Naphthalene 1,2-dioxygenase from Pseudomonas putida strain NCIB 9816-4 (NDO) is one of the most well studied Rieske dioxygenases; it is an α3β3 hexamer and is the first Rieske nonheme iron oxygenase for which the three-dimensional structure was determined. The α subunit of NDO contains a Rieske [2Fe–2S] center that accepts electrons from the ferredoxin component, which originate from an NAD(P)H on a reductase component, and transfers them to a nonheme mononuclear iron at the active site. The catalytic domain of the terminal oxygenase is the well described 2-His/carboxylate center composed of a mononuclear iron coordinated by two histidines and one aspartic acid inside a large hydrophobic active site. NDO has a relaxed substrate specificity and catalyzes the dioxygenation of many two-ring and three-ring aromatic compounds to their respective cis-dihydrodiols.

In order to study inhibition of the activity of NDO by inhibitory compounds, we also complexed NDO with the known inhibitors indole-3-acetate and benzamide and determined the structures of these complexes. The structure of NDO in complex with benzamide was determined to 1.65 Å resolution. Benzamide does bind in one orientation in the active site of NDO. It was hypothesized that this compound should bind tightly with the heteroatoms near the mononuclear iron because the aromatic ring could be positioned between Val209 and Leu307. In addition, the amide group would be able to interact with charged residues on the wall of the active site, while forming hydrogen bonds to the water/hydroxide bound to the mononuclear iron. The N atom of the substrate forms a hydrogen bond to the water/hydroxide that is bound to the mononuclear iron. The O atom of the inhibitor interacts with the side-chain N atom of Asn201, which is 3.6 Å away, and the side-chain N atom of Asn297, which is 4.0 Å away. There are no examples of NDO catalyzing the oxidation of compounds containing an amide group and it is unlikely, based on structural evidence, that NDO would be able to catalyze the oxidation of substrates with amide groups that are free to interact with the mononuclear iron very efficiently.

> MNYNNKILVSESGLSQKHLIHGDEELFQHELKTIFARNWLFLTHDSLIPAPGDYVTAKMGIDEVIVSRQNDGSIRAFLNVCRHRGKTLVSVEAGNAKGFVCSYHGWGFGSNGELQSVPFEKDLYGESLNKKCLGLKEVARVESFHGFIYGCFDQEAPPLMDYLGDAAWYLEPMFKHSGGLELVGPPGKVVIKANWKAPAENFVGDAYHVGWTHASSLRSGESIFSSLAGNAALPPEGAGLQMTSKYGSGMGVLWDGYSGVHSADLVPELMAFGGAKQERLNKEIGDVRARIYRSHLNCTVFPNNSMLTCSGVFKVWNPIDANTTEVWTYAIVEKDMPEDLKRRLADSVQRTFGPAGFWESDDNDNMETASQNGKKYQSRDSDLLSNLGFGEDVYGDAVYPGVVGKSAIGETSYRGFYRAYQAHVSSSNWAEFEHASSTWHTELTKTTDR;> MMINIQEDKLVSAHDAEEILRFFNCHDSALQQEATTLLTQEAHLLDIQAYRAWLEHCVGSEVQYQVISRELRAASERRYKLNEAMNVYNENFQQLKVRVEHQLDPQNWGNSPKLRFTRFITNVQAAMDVNDKELLHIRSNVILHRARRGNQVDVFYAAREDKWKRGEGGVRKLVQRFVDYPERILQTHNLMVFL> MHHHHHHGSGQRWELALGRFLEYLSWVSTLSEQVQEELLSSQVTQELRALMDETMKELKAYKSELEEQLTPVAEETRARLSKELQAAQARL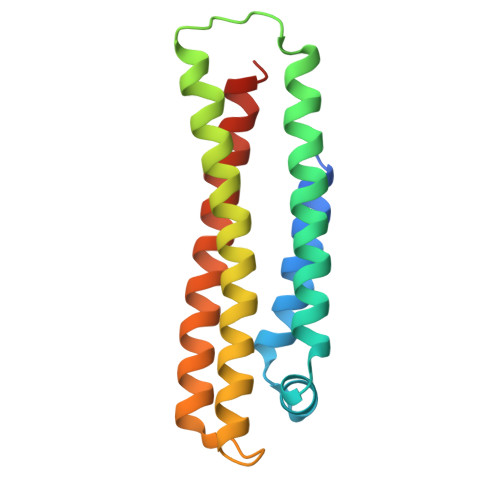GADMEDVRGRLVQYRGEVQAMLGQSTEELRVRLASHLIALQLRLIGDAFDLQKRLAVYQAGAAEQ> GSDASIDYNNKKSIIKKMYIFRYLTDKQCNLLIEAFRTTRYEEGDYIIQEGEVGSRFYIIKNGEVEIVKNKKRLRTLGKNDYFGERALLYDEPRTASVISKVNNVECWFVDKSVFLQIIQGPMLAHLEERIKMQDTKVEMDELE

Recent studies discovered that the P. falciparum cGMP-dependent protein kinase (PfPKG) is involved in both asexual and sexual development and specific inhibition of PfPKG blocked progression of the life cycle at multiple stages. PfPKG contains an N-terminal regulatory (R) domain including a possible auto-inhibitory (AI) sequence and a C-terminal catalytic (C) domain. Moreover, the R-domain of PfPKG contains four consensus cyclic nucleotide-binding domains (PfCNB-A, B, C and D), whereas mPKG has only two (mCNB-A and B). Cyclic GMP binding to PfCNB-D has been shown to have the greatest effect on kinase activation.

The final model containing residues 403–526 shows four ordered sulfate ions, with one of the sulfates occupying the cyclic phosphate site due to a high sulfate concentration in the crystallizing condition. The N-terminal portion of the αC-helix (residues 520–526) forms a loop, providing crystal contacts with the PBC of the neighboring molecule in the crystal lattice. The rest of the αC-helix (residues 527–542) is not modeled due to the lack of electron density. The αC-helix is not ordered in the absence of cGMP, but becomes ordered upon binding cGMP and shields the cGMP pocket. In the absence of cGMP, the PBC is open with its αP-helix positioned away from the -barrel. The αB-helix, which interacts directly with the PBC, is tilted away from the -barrel. The α310-helix of the N3A motif interacts directly with the PBC. Three phenylalanines from different regions, F419 (α310-helix), F434 (αA-helix) and F455 (3), together with the hinge residues, L486 (αP-helix) and F513 (αB-helix) as previously defined in the CNB domain of Epac2, form a hydrophobic core that stabilizes the apo conformation.>GAMSQDDDYLYCEKCQNFFIDSCPNHGP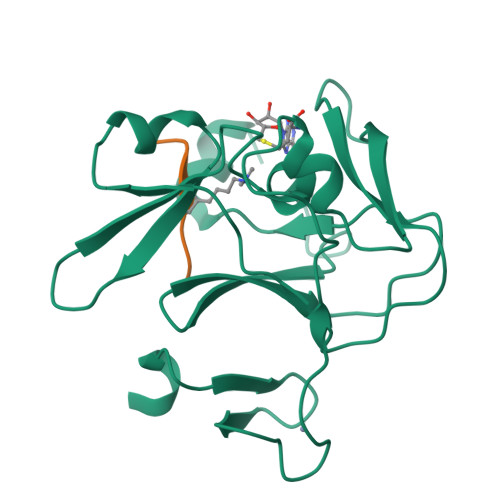PLFVKDSMVDRGHPNHSVLSLPPGLRISPSGIPEAGLGVWNEASDLPVGLHFGPYEGQITEDEEAANSGYSWLITKGRNCYEYVDGQDESQANWMRYVNCARDDEEQNLVAFQYHRKIFYRTCRVIRPGCELLVWYGDEYGQELGIK[2x];> ARTKQTARKY>GPGSMVVKRVFLSSDHAGVELRLFLSAYLRDLGCEVFDCGCDPKEHSVDYPDYVHDVVREVSDTSFGVLICGTGIGMSIAANRHKNIRAALCSSTMLAKLSREHNDANV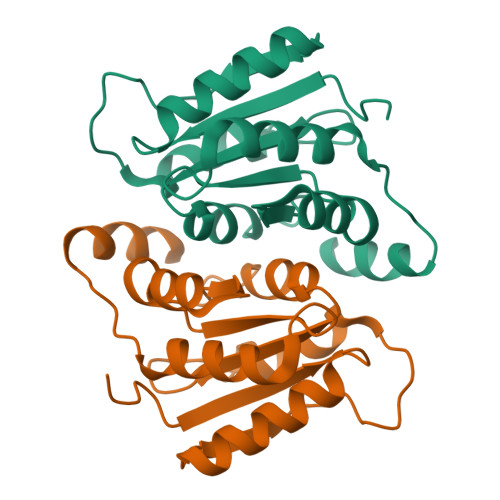LCFGSRYIDPDTAQSVLYTFMTTAFLGGRHAVRVQKLGE[2x]>[4x]ATQGVFT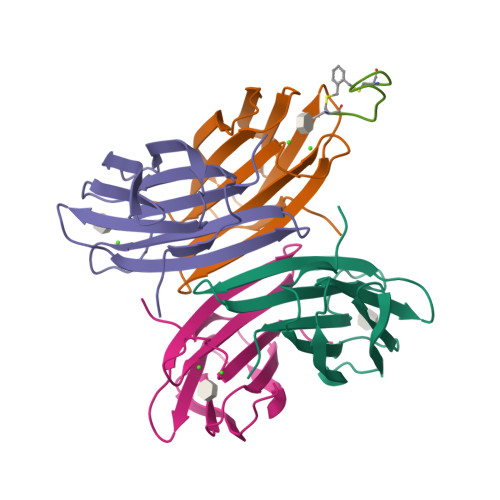LPANTRFGVTAFANSSGTQTVNVLVNNETAATFSGQSTNNAVIGTQVLNSGSSGKVQVQVSVNGRPSDLVSAQVILTNELNFALVGSEDGTDNDYNDAVVVINWPLG;> CWWKKKKKWWCA Variable temperature solution light scattering and/or SAXS experiments have provided important findings about influence of temperature on protein shape or association levels which expand our understanding. Previously, we provided a detailed structural and mechanistic insight of thermophilic l-asparaginase from Pyrococcus furiosus in its full-length (PfA), and a conjoined functional version (cPfA) (domain architecture shown in Supplementary Fig. S1). SAXS and crystal diffraction data analysis brought forth that despite lacking a 19-residue long linker which connects the two domains, namely the N- and C-halves (N-PfA and C-PfA, respectively), cPfA adopts a solution shape and crystalline state that is comparable to wild type full-length protein PfA with improved specific-activity. In conclusion, the findings reported here provide structural evidence in support of temperature induced higher order oligomer formation conferring stability to thermophilic proteins thereby regulating their functioning.

To visualize the structural changes accompanying PfA under high temperature conditions, crystallization was setup between 30 and 50 °C. However, no crystals were produced under these conditions. Since the residues involved in interactions (described above) were also present in the linker-less PfA variant cPfA, we attempted to crystallize the latter under high temperature conditions. Therefore, to get the structural insights into the oligomeric forms, we attempted crystallization of the cPfA at higher temperature. Detailed analysis showed negligible structural differences between both the structures (R.M.S.D at Cα, 0.12 Å). Thus, an increase in temperature had negligible effect on its structure. Furthermore, the symmetry-based N-terminal domains were bound by similar interactions as present at 18 °C. The absence of linker in this protein might have provided more flexibility in the alignment of N- and C-domains within the functional dimer assembly and as a result, the interactions between the N-N′ domains of different functional dimers became much stronger. The interaction analysis showed that 2 salt bridges, 8 H-bonds and 86 hydrophobic interactions were present between these domains. Residues R175 and D178, reversibly formed a salt bridge while G134, T168, E177, L179, V181 and N182 were involved in hydrogen bond formation. Importantly, as compared to PfA, cPfA had double the number of inter-chain H-bonds and hydrophobic interactions, implying that the N-terminal domains of cPfA were more strongly associated with each other.

> MKILLIGMGGTIASVKGENGYEASLSVKEVLDIAGIKDCEDCDFLDLKNVDSTLIQPEDWVDLAETLYKNVKKYDGIIVTHGTDTLAYTSSMISFMLRNPPIPIVFTGSMIPATEENSDAPLNLQTAIKFATSGIRGVYVAFNGKVMLGVRTSKVRTMSRDAFESINYPIIAELRGEDLVVN;> MAVLVIKLIPGLSGDIFRAAVELGYRGIVIEGYGAGGIPYRGSDLLQTIEELSKEIPIVMTTQAMYDGVDLTRYKVGRLALRAGVIPAGDMTKEATVTKLMWILGHTNNVEEIKVLMRKNLVGELRD>[4x]KIKVDELPVPEKFKEVLKSEGVRELLPVQSLAVKNGLLDGENLLVVSATASGKTLIGELAGVPKAMQGKKLLFLVPLVALANQKYEDFKRRYSKLGLRVAIRVGMSRIKTKDELVVVDTGIDADIIVGTYEGIDYLLRAGRKIGNVGTIVIDEIHTLDDEERGPRLDGLIARLRKLYPKAQFIGLSATVGNPDELAKELGLKLVLYDERPVDLERHIIIVRNESEKWRHIANLCRAEAMRKSKQGYKGQSIVFTFSRKRTHELAAYLTSKGLKAKPYHSGLPYKQRKLTEMEFLAQRLDVVVTTAALGAGVDFPASQVIFESLAMGNKWLSVREFHQMLGRAGRPLYHEKGKVYLLVEPGRKYSAQMEGTEDEVAFKLLTAPIEPVQVEWSDELEQDNVLAH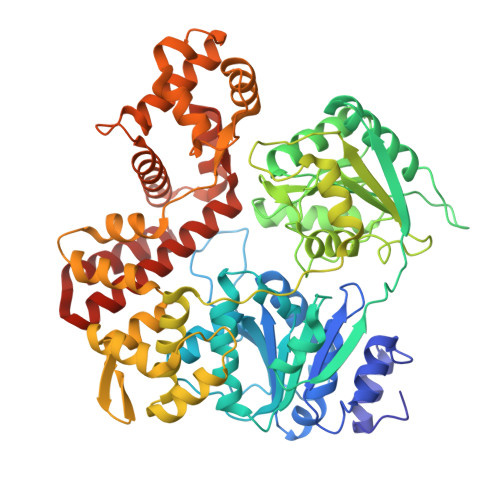SCVFNRLDVIEEVQSMCLGANQSAEKVLEKLEEFDFVKMKRPIVEVTPYGRAVSMSFLLPKEATFIRGNLGKREARWIAVKLLPFENIYLSGTLQRELEGAVRGRLSANVFSPSFASILEELDKVIPELSPNAAERLFTIYQEFFMCPEEDCTEYAMERVSNLIIELRRSGKHPTQIAEHFRKVYGLIVYPGDVFTWLDGIVRKLEAIERIARVFRVRKTEEGAKILKREIEEGRMI> MAHHHHHHVDDDDKMVLNFEEYKHTYFKSIKKGGIDWSLFPMKLYQLGKKLFWDPSTIDLTQDRADWDKLRDIDKFLMVNVTSKFGAGEEAVALDLHPLIVTLVKEGRVEEVMYLEQFIFEEAKHVEAFRRFLDAVGVKEDLVELTKDVSPNYAKIFYEELPKAMWNLNRDPSPENQVRAAVTYNLVVEGVAAEGGYNIFKYITRTFNIFPGLAKMVNYIATDESRHIAFGTYLIARLIKEGGESVYK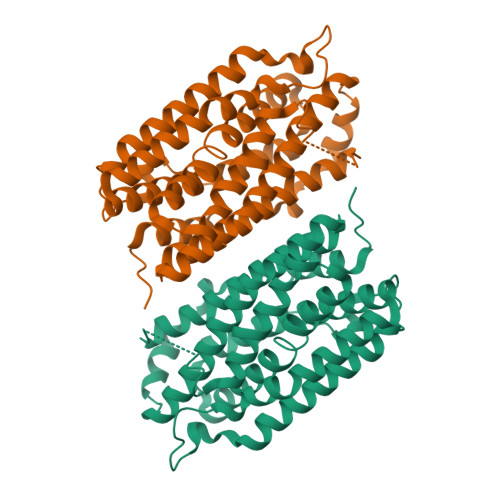AAMEHINYLGPYAVGIFSEPNVPQGVEIPLKLNPEVTVEYAKKLLNVRIQAIQRAKELKLEMLTPKDLDVIESL MyD88 and MAL are Toll-like receptor (TLR) adaptors that signal to induce pro-inflammatory cytokine production. We previously observed that the TIR domain of MAL (MALTIR) forms filaments in vitro and induces formation of crystalline higher-order assemblies of the MyD88 TIR domain (MyD88TIR). Here, we present MicroED and SFX structures of the MyD88TIR assembly, which reveal a two-stranded higher-order assembly arrangement of TIR domains analogous to that seen previously for MALTIR. We demonstrate via mutagenesis that the MyD88TIR assembly interfaces are critical for TLR4 signaling in vivo, and we show that MAL promotes unidirectional assembly of MyD88TIR.

Here we present MicroED and SFX structures of the MAL-induced MyD88TIR microcrystals at 3.0 Å and 2.3 Å resolution, respectively. The higher-resolution SFX structure (2.3 Å) was first solved using the MicroED MyD88TIR model as a template for molecular replacement followed by iterative rebuilding and refinement using a different protocol compared to the MicroED structure (SFXa). The SFXa map showed well-resolved features, including water molecules that were not modelled in the MicroED structure. The MyD88TIR SFXa structure was used for the comparison with other TIR domain structures and for the analyses of interaction interfaces within the crystal. The structure of MyD88TIR within the MAL-induced higher-order assembly exhibited conformational differences from the known NMR (RMSD of 2.4 Å for 107 Cα atoms)61 and X-ray (RMSD of 2.0 Å for 118 Cα atoms)62 structures of monomeric MyD88TIR. This is especially apparent in the region encompassing the BB loop and αB helix, and in the CD loop. Analysis of the crystal packing reveals MyD88TIR higher-order assemblies, each consisting of two offset parallel strands of TIR domains, with subunits in a head-to-tail arrangement forming each strand. Based on the SFX structure, the intrastrand interface involves opposite sides of the MyD88TIR domain, which together buries ~18.0–18.6% (1500 Å2) of the total surface area per subunit in the structure. It is composed of interactions between residues located in the BB loop of one subunit (BB surface) and the βD and βE strands and the αE helix on the next subunit (EE surface). The interstrand interface buries ~12.0–12.2% of the total surface area per subunit (991 Å2) and is composed of interactions between residues located on the αB and αC helices of one molecule (BC surface) and the CD loop and the αD helical region of the partner molecule (CD surface).

> ERFDAFICYCPSDIQFVQEMIRQLEQTNYRLKLCVSDRDVLPGTCVWSIASELIEKRCRRMVVVVSDDYLQSKECDFQTKFALSLSPGAHQKRLIPIKYKAMKKEFPSILRFITVCDYTNPCTKSWFWTRLAKALSLP> DMPVERILEAELAVEPDPVTNICQAADKQLFTLVEWAKRIPHFSELPLDDQVILLRAGWN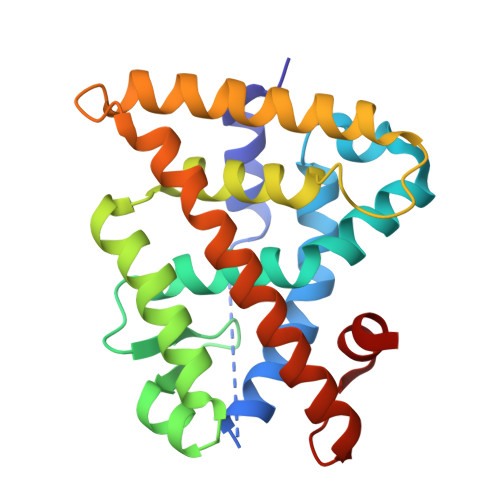ELLIASFSHRSIAVKDGILLATGLHVHRNSAHSAGVGAIFDRVLTELVSKMRDMQMDKTELGCLRAIVLFNPDSKGLSNPAEVEALREKVYASLEAYCKHKYPEQPGRFAKLLLRLPALRSIGLKCLEHLFFFKLIGDTPIDTFLMEMLE>MKQTLLLVEDDKNLADGLLVSLEQAGYECLHVERIADVEPQWKKADLVILDRQLPDGDSVQHLPEWKKIKDVPVILLTALVTVKDKVAGLDSGANDYLTKPFAEAELFARIRAQLRAPDSADQANADKVMTKDLEIDRATREVIFKGDLITLTRTEFDLLLFLASNLGRVFTRDELLDHVWGYNHFPTTRTVDTHVLQLRQKLPGLEIETLRGVGYK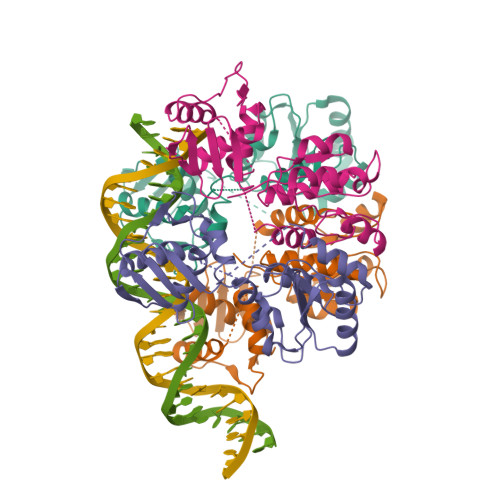MKA[8x]>[2x]MPPIIKRRVMRKIIIASQNPAKVNAVRSAFSTVFPDQEWEFIGVSVPSEVADQPMSDEETKQGALNRVRNAKQRHPGAEYYVGLEAGI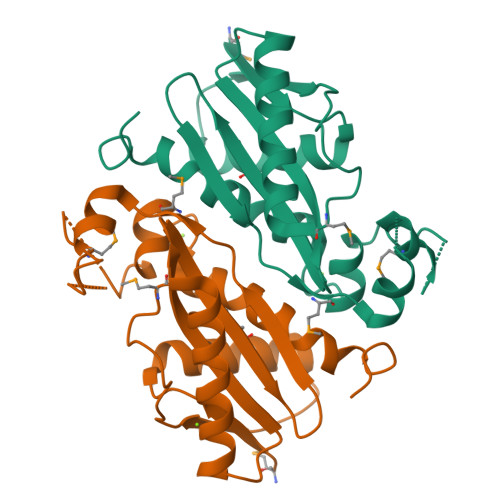EENKTFAWMIVESDQQRGESRSACLMLPPLVLERLRQAKELGDVMDEVFGTENIKQKGGAIGLLTRHHLTRSTVYHQALILALIPFINPEHYPSA>DPDPSQLHRSSLVKNLQNIYFLYEGDPVTHENVKSVDQLLSHDLIYNVSGPNYDKLKTELKNQEMATLFKDKNVDIYGVEYYHLCYLCENAERSACIYGGVT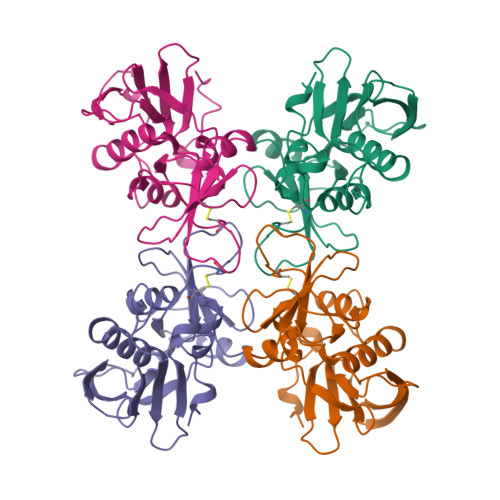NHEGNHLEIPKKIVVKVSIDGIQSLSFDIETNKKMVTAQELDYKVRKYLTDNKQLYTNGPSKYETGYIKFIPKNKESFWFDFFPEPEFTQSKYLMIYKDNETLDSNTSQIEVYLTTK[4x]> KDAVLVNSELKNIYMKDVINKTNMKITKKIGTQLIFNTNEKTRVWDDDNYNKVISS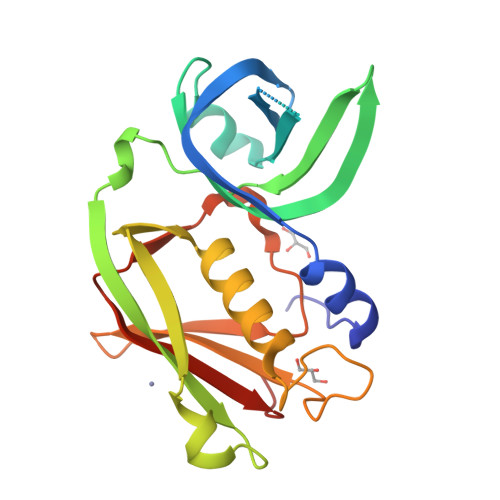NVSPAQERRFKEEEEVDIYALIKSYSVICKEQYNYVDGGLIKTSDREKLDSTIYMNIFGEQIPLKEQSKYKITFQNKFVTFQEIDVRLRKSLMSDNRIKLYEHNSICKKGYWGIHYKDNTTKFTDLFTHPNYTDNETIDMSKVSHFDVYLNEEFSKN> MRILAIDTATEACSVALWNNGTINAHFELCPREHTQRILPMVQEILAASGASLNEIDALAFGRGPGSFTGV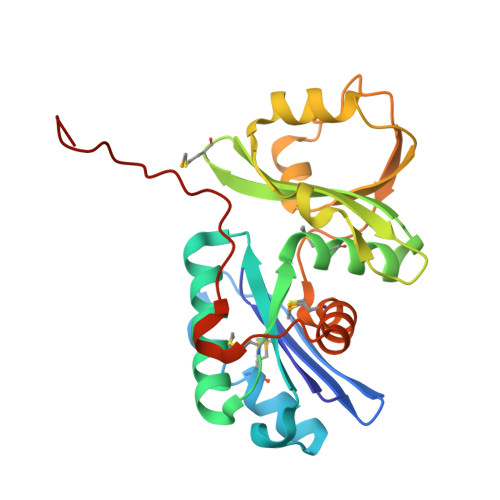RIGIGIAQGLALGANLPMIGVSTLATMAQGAWRKTGATRVLAAIDARMGEVYWAEYQRDAQGVWQGEETEAVLKPERVGERLKQLSGEWATVGTGWSAWPDLAKECGLTLHDGEVSLPAAEDMLPIASQKLAAGETVAVEHAEPVYLRNEVAWKKLPGKE> MVARPKSEDKKQALLEAATQAIAQSGIAASTAVIARNAGVAEGTLFRYFATKDELINTLYLHLYQDHCQSLIMELDRSITDAKMMIRFTWNSYISWGLNHP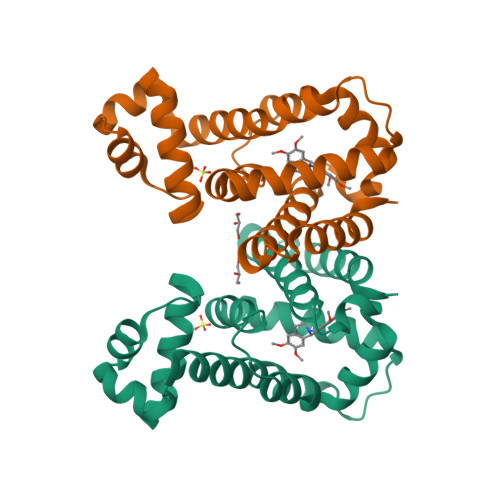ARHRAIRQLAVSEKLTKETKQRIEDMFPELRDILHRSVLMVFMSDEYSAFGKGLFYALAETTMDFAARDPARAGEYIALGFEAMWRALTREEQ>[4x]MRKLNPALEFRDFIQVLKDEDDLIEITEEIDPNLEVGAIMRKAYESHLPAPLFKNLKGASKDLFSILGCPAGLRSKEKGDHGRIAHHLGLDPKTTIKEI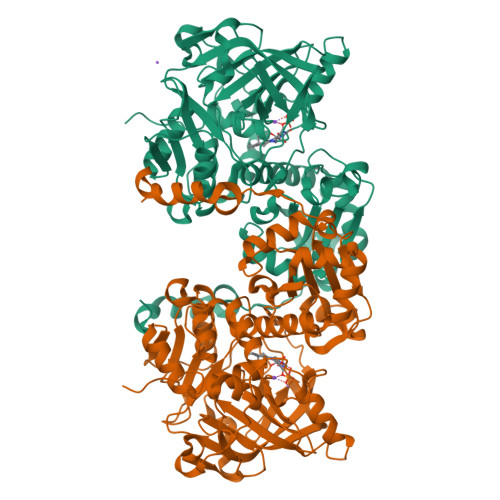IDYLLECKEKEPLPPITVPVSSAPCKTHILSEEKIHLQSLPTPYLHVSDGGKYLQTYGMWILQTPDKKWTNWSIARGMVVDDKHITGLVIKPQHIRQIADSWAAIGKANEIPFALCFGVPPAAILVSSMPIPEGVSESDYVGAILGESVPVVKCETNDLMVPATSEMVFEGTLSLTDTHLEGPFGEMHGYVFKSQGHPCPLYTVKAMSYRDNAILPVSNPGLCTDETHTLIGSLVATEAKELAIESGLPILDAFMPYEAQALWLILKVDLKGLQALKTTPEEFCKKVGDIYFRTKVGFIVHEIILVADDIDIFNFKEVIWAYVTRHTPVADQMAFDDVTSFPLAPFVSQSSRSKTMKGGKCVTNCIFRQQYERSFDYITCNFEKGYPKGLVDKVNENWKRYGYK> MNPIHDRTSDYHKYLKVKQGDSDLFKLTVSDKRYIWYNPDPDERDSYECGEIVSETSDSFTFKTVDGQDRQVKKDDANQRNPIKFDGVEDMSELSYLNEPAVFHNLRVRYNQDLIYTYSGLFLVAVNPFKRIPIYTQEMVDIFKGRRRNEVAPHIFAISDVAYRSMLDDRQNQSLLITGESGAGKTENTKKVIQYLASVAGRNQANGSGVLEQQILQANPILEAFGNAKTTRNNNSSRFGKFIEIQFNNAGFISGASIQSYLLEKSRVVFQSETERNYHIFYQLLAGATAEEKKALHLAGPESFNYLNQSGCVDIKGVSDEDEFKITRQAMDIVGFSQEEQMSIFKIIAGILHLGNIKFEKGAGEGAVLKDKTALNAASTVFGVNPSVLEKALMEPRILAGRDLVAQHLNVEKSSSSRDALVKALYGRLFLWLVKKINNVLCSERAAYFIGVLDISGFEIFKVNSFEQLCINYTNEKLQQFFNHHMFKVEQEEYLKEKINWTFIDFGLDSQATIDLIDGRQPPGILALLDEQSVFPNATDNTLITKLHSHFSKKNAKYEEPRFSKTEFGVTHYAGQVMYEIQDWLEKNKDPLQQDLELCFKDSSDNVVTKLFNDPNIASRAKKGANFITVAAQYKEQLASLMATLETTNPHFVRCIIPNNKQLPAKLEDKVVLDQLRCNGVLEGIRITRKGFPNRIIYADFVKRYYL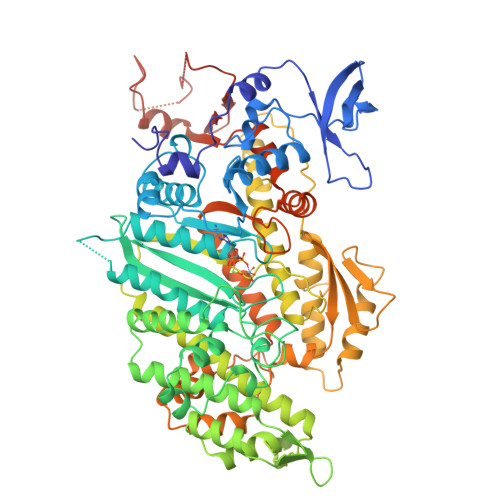LAPNVPRDAEDSQKATDAVLKHLNIDPEQYRFGITKIFFRAGQLARIEEARELPN>MTVPIAIIGTGIAGLSAAQALTAAGHQVHLFDKSRGSGGRMSSKRSDAGALDMGAQYFTARDRRFATAVKQWQAQGHVAEWTPLLYNFHAGRLSPSPDEQVRWVGKPGMSAITRAMRGDMPVSFSCRITEVFRGEEHWNLLDAEGQNHGPFSHVIIATPAPQASTLLAAAPKLASVVAGVKMDPTWAVALAFETPLQTPMQGCFVQDSPLDWLARNRSKPERDDTLDTWILHATSQWSRQNLDASREQVIEHLHGAFAELIDCTMPAPVFSLAHRWLYARPAGAHEWGALSDADLGIYVCGDWCLSGRVEGAWLSGQEAARRLLEHLQL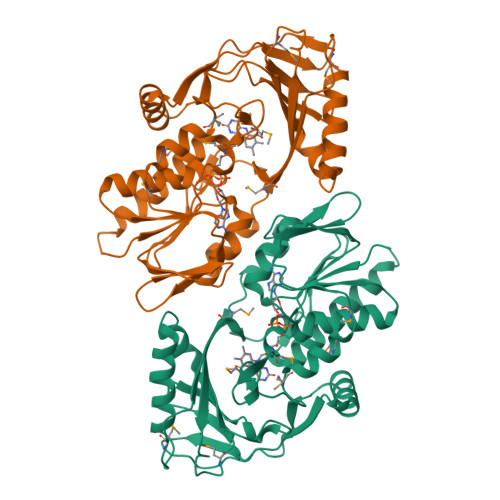EHHHHHH[2x]>MAVVFVNKLTLIGDAEEFESRYEAVGAFMETQPGLVRYSLVRSTKDDSVYFNIAEWDDEDTFRKALAEPE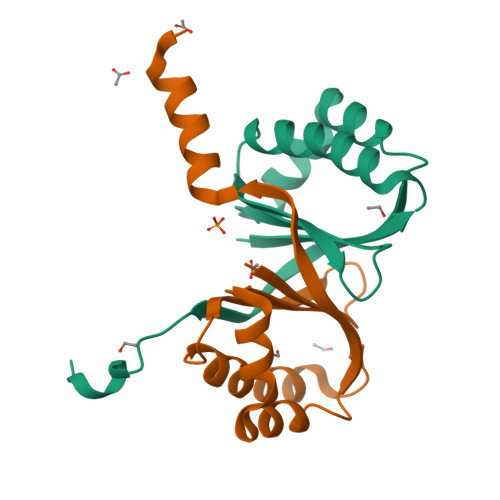FRRRLDALTGLIKGEPHLSLPVRQGRAAQVLENLYFQGHHHHHH[2x]>GSGAD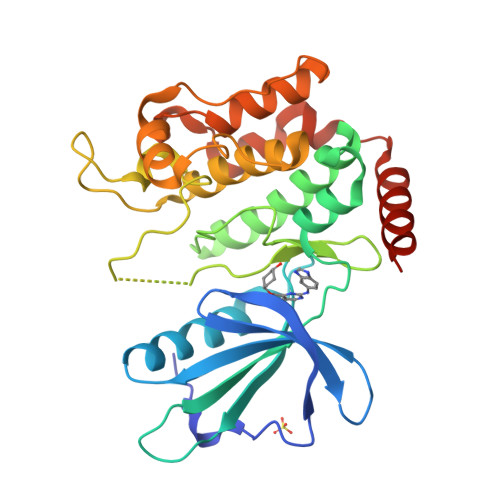EIDLSALRDPAGIFELVELVGNGTYGQVYKGRHVKTGQLAAIKVMDVTGDEEEEIKQEINMLKKYSHHRNIATYYGAFIKKNPPGMDDQLWLVMEFCGAGSVTDLIKNTKGNTLKEEWIAYICREILRGLSHLHQHKVIHRDIKGQNVLLTENAEVKLVDFGVSAQLDRTVGRRNTFIGTPYWMAPEVIACDENPDATYDFKSDLWSLGITAIEMAEGAPPLCDMHPMRALFLIPRNPAPRLKSKKWSKKFQSFIESCLVKNHSQRPATEQLMKHPFIRDQPNERQVRIQLKDHIDRTKKKRG[3x]>[2x]SNAMDKFLITGGVKLEGEVRISGAKNAALPLLAAMILADSPITLTNVPNLKDVNTLVKLIGGLGVTISYENDTVKADTSTLDNQFAPYELVKTMRASILVLGPLLARYGNAKVSLPGGCAIGSRPVDQHLKALEALGAHIEVENGYVHATVDGRLKGGEVVFDMVTVGGTENILMA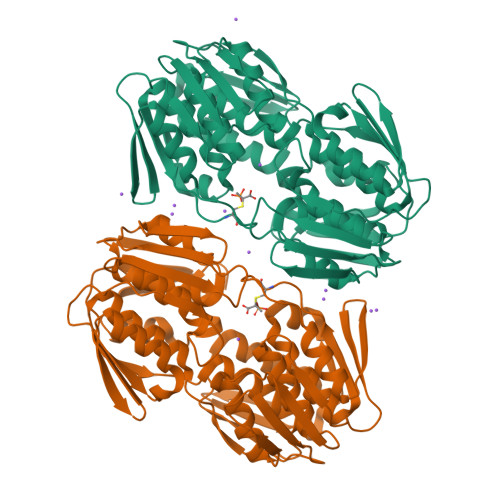AALADGVTTIRNAAREPEITDLAQMLIKMGAKIEGLDTDTLVVTGVESLHGCEYAVVADRIETGSYLAAAAITGGRVKTTHTDPSLLEAVLDKFEEMGAEVTRGDDWIELDMLGKRPKAVSFRTLPHPEFPTDMQAQIMAVNAIGRGFATISETIFENRFMHVPELSRMGANIQVEGHDAVVTGVEKLQAAPVMATDLRASFSLVLAALVAEGDTLIDRIYHIDRGYEHVEEKLQGLGAKIKRVS>MHNVLIVGASRGIGLGLADAFLQRGAQVFAVARRPQGSPGLQALAERAGERLQAVTGDLNQHDCAERIGEMLGERRIDRLIVNAGIYGPQQQDVAEIDAEQTAQLFLTNAIAPLRLARALSGRVSRGGVVAFMSSQMASLALG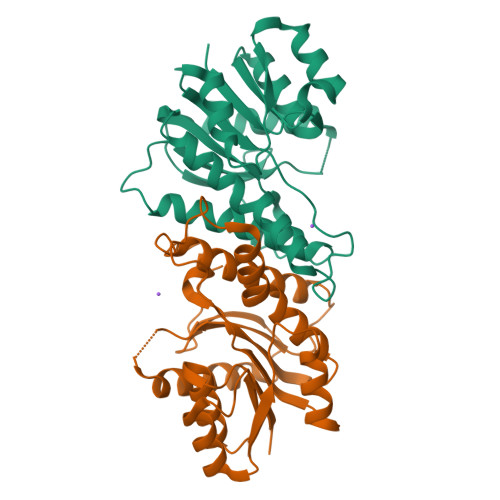LSATMPLYGASKAALNSLVRSWEGEFEELPFSLLLLHPGWVRTEMGGDSAPLSVEESAAGLVAAVEDAAGVNACRFVDYRNQPLPW[4x]> SALTPQLKDTLEKLVNSEKVVLFMKGTRDFPMCGFSNTVVQILKNLNVPFEDVNILENEMLRQGLKEYSNWPTFPQLYIGGEFFGGCDITLEAFKTGELQEEVEKAMCS

Arabidopsis chloroplastic Grx, AtGRXcp, was the first plant monothiol Grx to be characterized and plays an important role in redox regulation and protection against oxidative stress in chloroplasts. AtGRXcp is classified as a monothiol glutaredoxin with a CGFS active-site motif. Monothiol Grxs contain a single cysteine residue in the putative active-site motif CXXS and are conserved across species. It has been shown that monothiol Grxs have diverse biological functions such as protection against protein oxidation in chloroplasts, biogenesis of iron–sulfur clusters in mitochondria and regulation of iron homeostasis.

The crystal structure of AtGRXcp has been determined at 2.4 Å resolution. The structural model contains residues 65–173 of AtGRXcp, the chloroplastic signal peptide of which is removed. There is only one protein molecule in the crystallographic asymmetric unit. The structure of AtGRXcp has a glutaredoxin/thioredoxin-like fold with a core four-stranded parallel β-sheet flanked by five α-helices on both sides. A long groove is observed adjacent to Cys97 with a width of 11–14 Å and a length of 16–19 Å. The groove is formed by highly conserved residues present in plant monothiol Grxs and would be the binding site for glutathione (GSH), i.e. a γ-­Glu-Cys-Gly tripeptide. Structural comparative analysis shows that a glutathione molecule may fit into this groove, form a disulfide bond with the catalytic Cys97 and interact with several charged residues including Lys89, Arg126 and Asp152. In addition, comparative structural studies and sequence-alignment analysis of monothiol and dithiol Grxs reveal that monothiol Grxs (e.g. CGFS-type Grxs), with the exceptions of ScGrx6, ScGrx7 and GrxS12, have five additional amino acids (i.e. Thr91-Arg92-Asp93-Phe94-Pro95 in AtGRXcp) immediately upstream of the active-site Cys97. Most interestingly, similar to dithiol Grxs, ScGrx6, ScGrx7 and GrxS12 lack these five amino-acid residues and are also active in hydroxyethyl disulfide HEDS assays and have GSH-dependent oxido­reductase activity. This long unique loop with five additional residues adjacent to the catalytic Cys97 may be a key structural feature of monothiol Grxs.2'-DEOXY-GUANOSINE | C10 H13 N5 O4 | 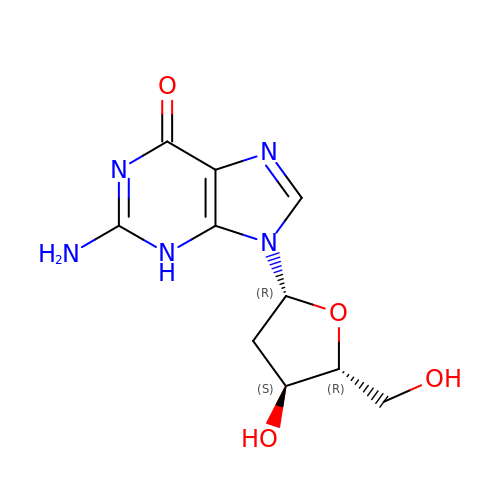YKBGVTZYEHREMT-KVQBGUIXSA-N5-FLUORO-2,6-DIOXO-1,2,3,6-TETRAHYDROPYRIMIDINE-4-CARBOXYLIC ACID | C5 H3 F 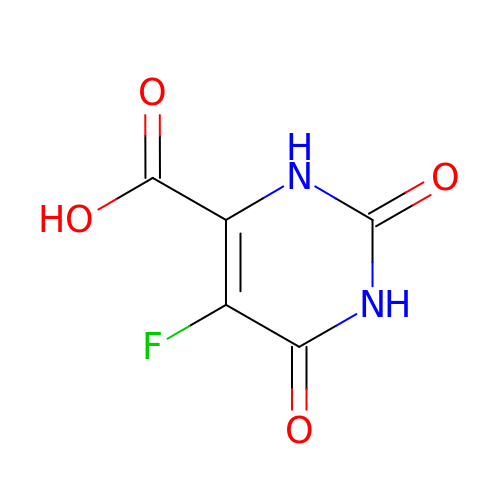N2 O4 | SEHFUALWMUWDKS-UHFFFAOYSA-N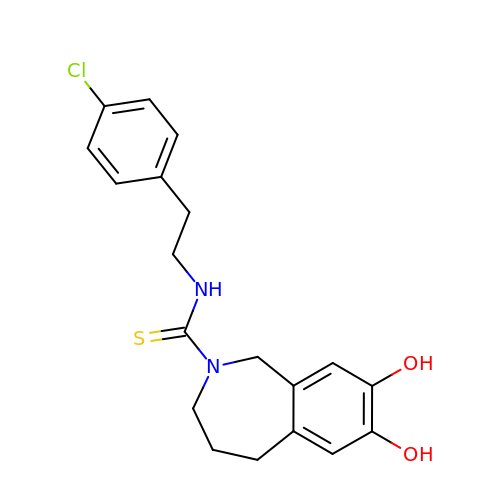capsazepine | C19 H21 Cl N2 O2 S | DRCMAZOSEIMCHM-UHFFFAOYSA-N>GSHMPNYDTSIDIEDIKKILPHRYPFLLVDKVIYMQPNKTIIGLKQVSTNEPFFNGHFPQKQIMPGVLQIEALAQLAGILCLKSDDSQKNNLFLFAGVDGVRWKKPVLP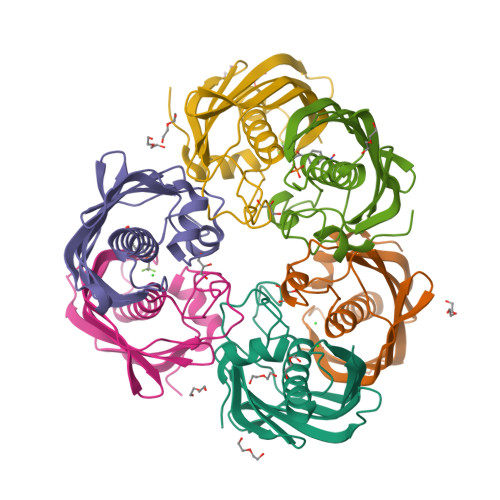GDTLTMQANLISFKSSLGIAKLSGVGYVNGKVVINISEMTFALSK[24x]> MLGTGPAAATTAATTSSNVSVLQQFASGLKSRNEETRAKAAKELQHYVTMELREMSQEESTRFYDQLNHHIFELVSSSDANERKGGILAIASLIGVEGGNATRIGRFANYLRNLLPSNDPVVMEMASKAIGRLAMAGDTFTAEYVEFEVKRALEWLGADRNEGRRHAAVLVLRELAISVPTFFFQQVQPFFDNIFVAVWDPKQAIREGAVAALRACLILTTQREPKEMQKPQWYRHTFEEAEKGFDETLAKEKGMNRDDRIHGALLILNELVRISSMEGERLREEMEEITQQQLVHDKYCKDLMGFGTKPRHITPFTSFQAVQPQQSNALVGLLGYSSHQGLMGFGTSPSPAKSTLVESRCCRDLMEEKFDQVCQWVLKCRNSKNSLIQMTILNLLPRLAAFRPSAFTDTQYLQDTMNHVLSCVKKEKERTAAFQALGLLSVAVRSEFKVYLPRVLDIIRAALPPKDFAHKRQKAMQVDATVFTCISMLARAMGPGIQQDIKELLEPMLAVGLSPALTAVLYDLSRQIPQLKKDIQDGLLKMLSLVLMHKPLRHPGMPKGLAHQLASPGLTTLPEASDVGSITLALRTLGSFEFEGHSLTQFVRHCADHFLNSEHKEIRMEAARTCSRLLTPSIHLISGHAHVVSQTAVQVVADVLSKLLVVGITDPDPDIRYCVLASLDERFDAHLAQAENLQALFVALNDQVFEIRELAICTVGRLSSMNPAFVMPFLRKMLIQILTELEHSGIGRIKEQSARMLGHLVSNAPRLIRPYMEPILKALILKLKDPDPDPNPGVINNVLATIGELAQVSGLEMRKWVDELFIIIMDMLQDSSLLAKRQVALWTLGQLVASTGYVVEPYRKYPTLLEVLLNFLKTEQNQGTRREAIRVLGLLGALDPYKHKVNIGMIDQSRDASAVSLSESKSSQDSSDYSTSEMLVNMGNLPLDEFYPAVSMVALMRIFRDQSLSHHHTMVVQAITFIFKSLGLKCVQFLPQVMPTFLNVIRVCDGAIREFLFQQLGMLVSFVKSHIRPYMDEIVTLMREFWVMNTSIQSTIILLIEQIVVALGGEFKLYLPQLIPHMLRVFMHDNSPGRIVSIKLLAAIQLFGANLDDYLHLLLPPIVKLFDAPEAPLPSRKAALETVDRLTESLDFTDYASRIIHPIVRTLDQSPELRSTAMDTLSSLVFQLGKKYQIFIPMVNKVLVRHRINHQRYDVLICRIVKGYTLADEEEDPLIYQHRMLRSGQGDALASGPVETGPMKKLHVSTINLQKAWGAARRVSKDDWLEWLRRLSLELLKDSSSPSLRSCWALAQAYNPMARDLFNAAFVSCWSELNEDQQDELIRSIELALTSQDIAEVTQTLLNLAEFMEHSDKGPLPLRDDNGIVLLGERAAKCRAYAKALHYKELEFQKGPTPAILESLISINNKLQQPEAAAGVLEYAMKHFGELEIQATWYEKLHEWEDALVAYDKKMDTNKDDPELMLGRMRCLEALGEWGQLHQQCCEKWTLVNDETQAKMARMAAAAAWGLGQWDSMEEYTCMIPRDTHDGAFYRAVLALHQDLFSLAQQCIDKARDLLDAELTAMAGESYSRAYGAMVSCHMLSELEEVIQYKLVPERREIIRQIWWERLQGCQRIVEDWQKILMVRSLVVSPHEDMRTWLKYASLCGKSGRLALAHKTLVLLLGVDPSRQLDHPLPTVHPQVTYAYMKNMWKSARKIDAFQHMQHFVQTMQQQAQHAIATEDQQHKQELHKLMARCFLKLGEWQLNLQGINESTIPKVLQYYSAATEHDRSWYKAWHAWAVMNFEAVLHYKHQNQARDEKKKLRHASGANITNATTAATTAATATTTASTEGSNS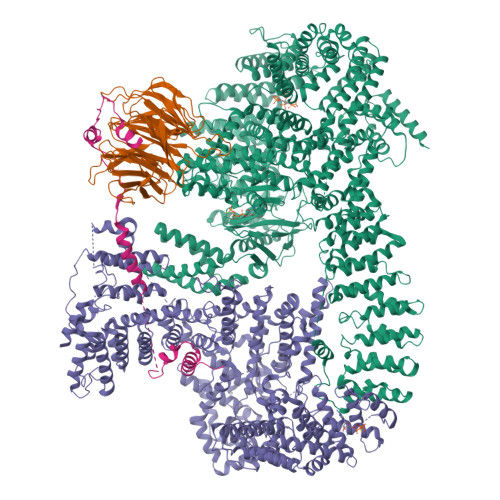ESEAESTENSPTPSPLQKKVTEDLSKTLLMYTVPAVQGFFRSISLSRGNNLQDTLRVLTLWFDYGHWPDVNEALVEGVKAIQIDTWLQVIPQLIARIDTPRPLVGRLIHQLLTDIGRYHPQALIYPLTVASKSTTTARHNAANKILKNMCEHSNTLVQQAMMVSEELIRVAILWHEMWHEGLEEASRLYFGERNVKGMFEVLEPLHAMMERGPQTLKETSFNQAYGRDLMEAQEWCRKYMKSGNVKDLTQAWDLYYHVFRRISKQLPQLTSLELQYVSPKLLMCRDLELAVPGTYDPNQPIIRIQSIAPSLQVITSKQRPRKLTLMGSNGHEFVFLLKGHEDLRQDERVMQLFGLVNTLLANDPTSLRKNLSIQRYAVIPLSTNSGLIGWVPHCDTLHALIRDYREKKKILLNIEHRIMLRMAPDYDHLTLMQKVEVFEHAVNNTAGDDLAKLLWLKSPSSEVWFDRRTNYTRSLAVMSMVGYILGLGDRHPSNLMLDRLSGKILHIDFGDCFEVAMTREKFPEKIPFRLTRMLTNAMEVTGLDGNYRITCHTVMEVLREHKDSVMAVLEAFVYDPLLNWRLMDTNTKGNKRSRTRTDSYSAGQSVEILDGVELGEPAHKKTGTTVPESIHSFIGDGLVKPEALNKKAIQIINRVRDKLTGRDFSHDDTLDVPTQVELLIKQATSHENLCQCYIGWCPFW;> MNTSPGTVGSDPVILATAGYDHTVRFWQAHSGICTRTVQHQDSQVNALEVTPDRSMIAAAGYQHIRMYDLNSNNPNPIISYDGVNKNIASVGFHEDGRWMYTGGEDCTARIWDLRSRNLQCQRIFQVNAPINCVCLHPNQAELIVGDQSGAIHIWDLKTDHNEQLIPEPEVSITSAHIDPDASYMAAVNSTGNCYVWNLTGGIGDEVTQLIPKTKIPAHTRYALQCRFSPDSTLLATCSADQTCKIWRTSNFSLMTELSIKSGNPGESSRGWMWGCAFSGDSQYIVTASSDNLARLWCVETGEIKREYGGHQKAVVCLAFNDSVLG;> MAAIGRGRSLKNLRVRGRNDSGEENVPLDLTREPSDNLREILQNVARLQGVSNMRKLGHLNNFTKLLCDIGHSEEKLGFHYEDIIICLRLALLNEAKEVRAAGLRALRYLIQDSSILQKVLKLKVDYLIARCIDIQQSNEVERTQALRLVRKMITVNASLFPSSVTNSLIAVGNDGLQERDRMVRACIAIICELALQNPEVVALRGGLNTILKNVIDCQLSRINEALITTILHLLNHPKTRQYVRADVELERILAPYTDFHYRHSPDTAEGQLKEDREARFLASKMGIIATFRSWAGIINLCKPGNSGIQSLIGVLCIPNMEIRRGLLEVLYDIFRLPLPVVTEEFIEALLSVDPGRFQDSWRLSDGFVAAEAKTILPHRARSRPDLMDNYLALILSAFIRNGLLEGLVEVITNSDDHISVRATILLGELLHMANTILPHSHSHHLHCLPTLMNMAASFDIPKEKRLRASAALNCLKRFHEMKKRGPKPYSLHLDHIIQKAIATHQKRDQYLRVQKDIFILKDTEEALLINLRDSQVLQHKENLEWNWNLIGTILKWPNVNLRNYKDEQLHRFVRRLLYFYKPSSKLYANLDLDFAKAKQLTVVGCQFTEFLLESEEDGQGYLEDLVKDIVQWLNASSGMKPERSLQNNGLLTTLSQHYFLFIGTLSCHPHGVKMLEKCSVFQCLLNLCSLKNQDHLLKLTVSSLDYSRDGLARVILSKILTAATDACRLYATKHLRVLLRANVEFFNNWGIELLVTQLHDKNKTISSEALDILDEACEDKANLHALIQMKPALSHLGDKGLLLLLRFLSIPKGFSYLNERGYVAKQLEKWHREYNSKYVDLIEEQLNEALTTYRKPVDGDNYVRRSNQRLQRPHVYLPIHLYGQLVHHKTGCHLLEVQNIITELCRNVRTPDLDKWEEIKKLKASLWALGNIGSSNWGLNLLQEENVIPDILKLAKQCEVLSIRGTCVYVLGLIAKTKQGCDILKCHNWDAVRHSRKHLWPVVPDDVEQLCNELSSIPSTLSLNSESTSSRHNSESESVPSSMFILEDDRFGSSSTSTFFLDINEDTEPTFYDRSGPIKDKNSFPFFASSKLVKNRILNSLTLPNKKHRSSSDPKGGKLSSESKTSNRRIRTLTEPSVDFNHSDDFTPISTVQKTLQLETSFMGNKHIEDTGSTPSIGENDLKFTKNFGTENHRENTSRERLVVESSTSSHMKIRSQSFNTDTTTSGISSMSSSPSRETVGVDATTMDTDCGSMSTVVSTKTIKTSHYLTPQSNHLSLSKSNSVSLVPPGSSHTLPRRAQSLKAPSIATIKSLADCNFSYTSSRDAFGYATLKRLQQQRMHPSLSHSEALASPAKDVLFTDTITMKANSFESRLTPSRFMKALSYASLDKEDLLSPINQNTLQRSSSVRSMVSSATYGGSDDYIGLALPVDINDIFQVKDIPYFQTKNIPPHDDRGARAFAHDAGGLPSGTGGLVKNSFHLLRQQMSLTEIMNSIHSDASLFLESTEDTGLQEHTDDNCLYCVCIEILGFQPSNQLSAICSHSDFQDIPYSDWCEQTIHNPLEVVPSKFSGISGCSDGVSQEGSASSTKSTELLLGVKTIPDDTPMCRILLRKEVLRLVINLSSSVSTKCHETGLLTIKEKYPQTFDDICLYSEVSHLLSHCTFRLPCRRFIQELFQDVQFLQMHEEAEAVLATPPKQPIVDTSAES;> AFLDNPTIILAHIRQSHVTSDDTGMCEMVLIDHDVDLEKIHPPSMPGDSGSEIQGSNGETQGYVYAQSVDITSSWDFGIRRRSNTAQRLERLRKERQNQIKCKNIQWKERNSKQSAQELKSLFEKKSLKEKPPISGKQSILSVRLEQCPLQLNNPFNEYSKFDGKGHVGTTATKKIDVYLPLHSSQDRLLPMTVVTMASARVQDLIGLICWQYTSEGREPKLNDNVSAYCLHIAEDDGEVDTDFPPLDSNEPIHKFGFSTLALVEKYSSPGLTSKESLFVRINAAHGFSLIQVDNTKVTMKEILLKAVKRRKGSQKVSGPQYRLEKQSEPNVAVDLDSTLESQSAWEFCLVRENSSRADGVFEEDSQIDIATVQDMLSSHHYKSFKVSMIHRLRFTTDVQLGISGDKVEIDPVTNQKASTKFWIKQKPISIDSDLLCACDLAEEKSPSHAIFKLTYLSNHDYKHLYFESDAATVNEIVLKVNYILESRASTARADYFAQKQRKLNRRTSFSFQKEKKSGQQ(4S)-1-methyl-4-(prop-1-en-2-yl)cyclohex-1-ene 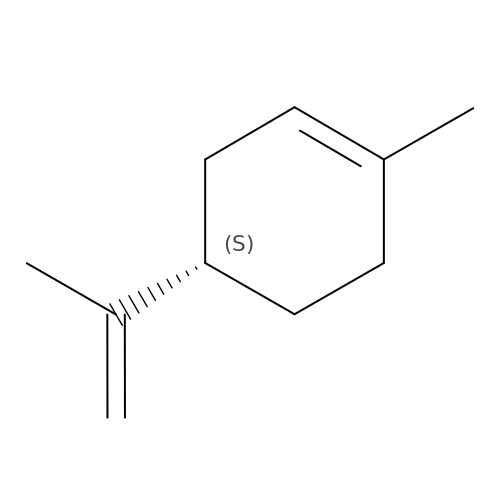| C10 H16 | XMGQYMWWDOXHJM-SNVBAGLBSA-N>[4x]HPETLVKVKDAEDQLGARVGYIELDLNSGKILESFRPEERFPMMSTFKVLLCGAVLSRVDAGQEQLGRRIHYSQNDLVEYSPVTEKHLTDGMTVRELCSAAITMSDNTAANLLLTTIGGPKELTAFLHNMGDHVTRLDRWEPELNEAIPNDERDT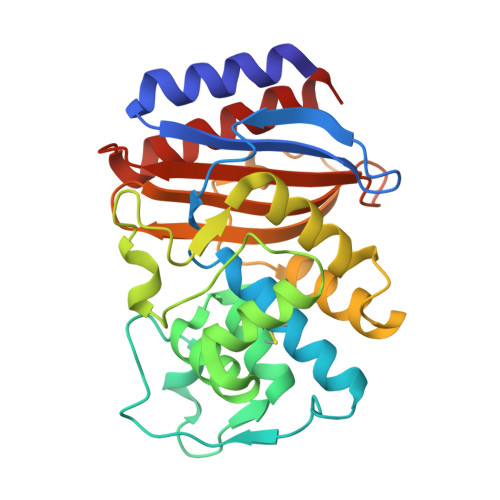TTPAAMATTLRKLLTGELLTLASRQQLIDWMEADKVAGPLLRSALPAGWFIADKSGAGERGSRGIIAALGPDGKPSRIVVAYTTGSQATMDERNRQIAEIGASLIKHW> MATAGNPWGWFLGYLILGVAGSLVSGSCSQIINGEDCSPHSQPWQAALVMENELFCSGVLVHPQWVLSAAHCFQNSYTIGLGLHSLEADQEPGSQMVEASLSVRHPEYNRPLLANDLMLIKLDESVSESDTIRSISIASQCPTAGNSCLVSGWGLLANGRMPTVLQCVNVSVVSEEVCSKLYDPLYHPSMFCAGGGHDQKDSCNGDSGGPLICNGYLQGLVSFGKAPCGQVGVPGVYTNLCKFTEWIEKTVQAS;> PQFGLFSKYRTPNCRRYSIH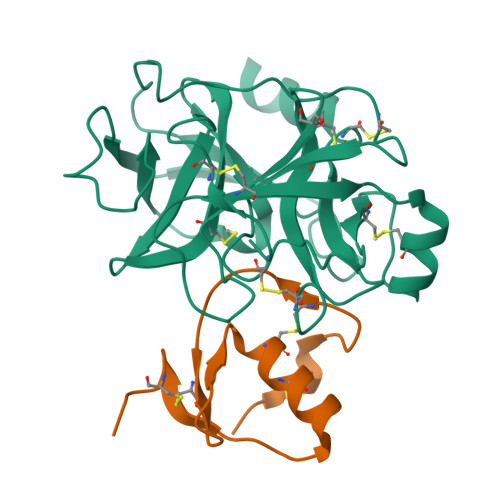GCNRMYAPVCGSDMSTYANECTLCMKIREGGHNIKIIKNGPCGAS> NNKTLAAMKNFAEQYAKRTDTYFCSDLSVTAVVIEGLARHKEELGSPLCPCRHYEDKEAEVKNTFWNCPCVPMRERKECHCMLFLTPDNDFAGD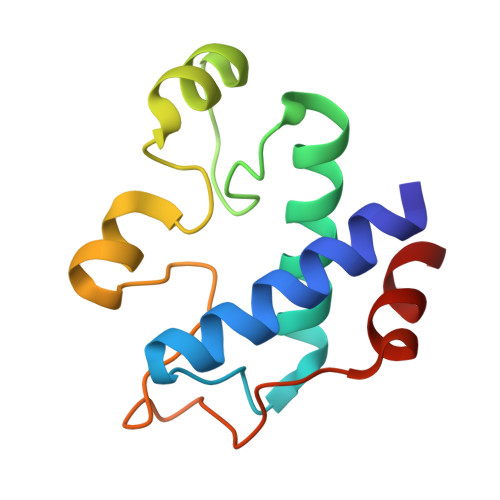AQDIPMETLEEVKAS>MPHLFDPYRIGNLELANRIAIAPMCQYSAQEGNATDWHMIHLGQMALSGAGLLIIEATAVSPEGRITPTDLGLYNDANEAALGRVLGAVRNHSPIAVTIQLAHAGRKASSEAPWDGGGQIRPDQPRGWQTFAPSAVPHAAGEVPPAALDKAGMKKIRDDFVAAAKRAARLGIEGIEVHGAHGYLLHQFLSPIANHRTDEYGGSLENRMRFPLEVFDAVREAFPAERPVWMRVSATDWVPNGWDIEGTIALSHELKARGSAAVHVSTGGVSPQQAIKIGPGYQVPYAQRVKAEV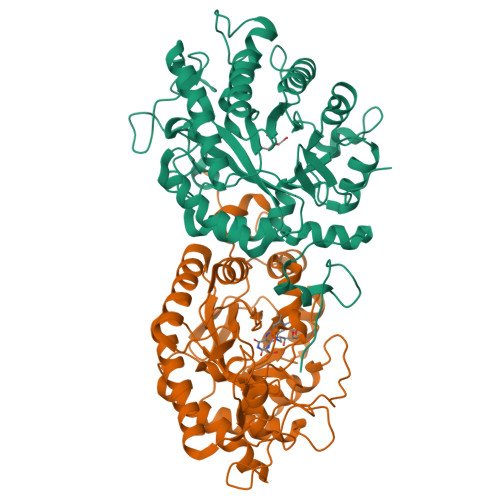GLPTMAVGLITEAEQAEAIIANNEADIISIARAMLYDPRWPWHAAAKLGASVNAPKQYWRSQPRGLEKLFKDAHFGQR[4x]>MVRVKICGITNLEDALFSVESGADYVGFVFYPKSKRYISPEDARRISVELPVERVGVFVNEEPEKILDVASYVQLNAVQLHGEEPIELCRKIAERILVWKAVGVSNERDMERALNYREFPILLDTKTPEYGGSGKTFDWSLILPYRDRFRYLVLSGGLNPENVRSAIDVVRPFAVDVS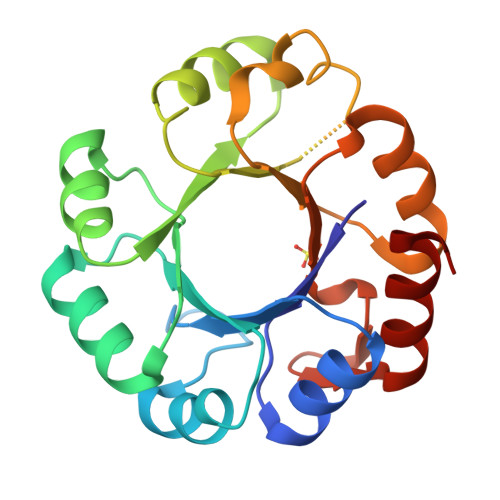SGVEAFPGKKDHDSIKMFIKNAKGL[2x]We previously synthesized an iodinated variant (7iGST) of eukaryotic glutathione S-transferase (GST), a homodimeric detoxification enzyme, in which seven specific residues of the 15 tyrosines per monomer were replaced by 3-iodo-l-tyrosines. The seven sites, specified with seven UAG codons in the gene, were distributed globally in the enzyme, including four on the surface (positions −1, 22, 141, and 163), two buried (positions 57 and 155), and one at the dimer interface (position 73). In the present study, two additional variants (7bGST and 7cGST), which contained 3-bromo- and 3-chlorotyrosines, respectively, in place of 3-iodotyrosine, were also synthesized in RFzero-iy, with these tyrosine derivatives being supplemented in the growth media. The structural study showed that the chlorination and bromination of the selected tyrosine residues achieved a more tightly packed protein interior, with the bulky atoms filling internal spaces and creating additional interresidue interactions.

The halogenation at position 32 significantly increased the heat resistance of 3bGST and 3cGST, whereas those at positions 27 and 56 each abolished the resistance. Finally, position 32 was halogenated and position 155 was made halogen-free in the initial variants 7bGST and 7cGST, to create 7bGST-1 and 7cGST-1, respectively. The heat resistance was drastically increased (0 to 71% for 7bGST-1, 11 to 79% for 7cGST-1), and was accompanied by significant recoveries of the specific activity (47 to 67% for 7bGST-1 and 60 to 72% for 7cGST-1). The ΔG(H2O) values for 7bGST-1 and 7cGST-1 (33.3 and 32.9 kcal/mol, respectively) were larger by 5.6 and 5.2 kcal/mol, respectively, than that of wtGST. The major stabilizing positions 32, 57, and 73 are located in domain I, which consists of a four-stranded β-sheet and three α-helices. The side chains of the halogenated tyrosines at positions 32 and 57 (Hal32 and Hal57) protrude from each side of the β-sheet, and are buried in the protein interior. The halogen moiety of Hal32 fills the space between the side chains of Lys39 and Lys43, while that of Hal57 fills the space between the side chains of Pro2, Leu4, Leu20, and Tyr27. The halogen moiety of Hal73 occupies the space at the dimer interface, between the side chains of Lys77 and Lys86, where Lys86 belongs to the other monomer. The halogen atoms are accommodated in spaces with sizes between 1.25 and 1.70 Å for wtGST, while the radii of the bromine and chlorine atoms are 1.85 and 1.75 Å, respectively. Thus, the bulky halogens do not simply occupy vacant spaces that are large enough for the atoms, but fit into the spaces by causing local structural changes, probably involving side-chain movements, which cannot be identified from the crystal structures with the present resolutions.

> MASMTGGQQMGRDPGANSGVTKNSXSPILGYWKIKGLVQPTRLLLEXLEEKYEEHLXERDEGDKWRNKKFELGLEFPNLPYXIDGDVKLTQSMAIIRXIADKHNMLGGCPKERAEISMLEGAVLDIRYGVSRIAYSKDFETLKVDFLSKLPEMLKMFEDRLCHKTXLNGDHVTHPDFMLYDALDVVLXMDPMCLDAFPKLVCFKKRIEAIPQIDKYLKSSKYIAWPLQGWQATFGGGDHPPKSD>[2x]IQT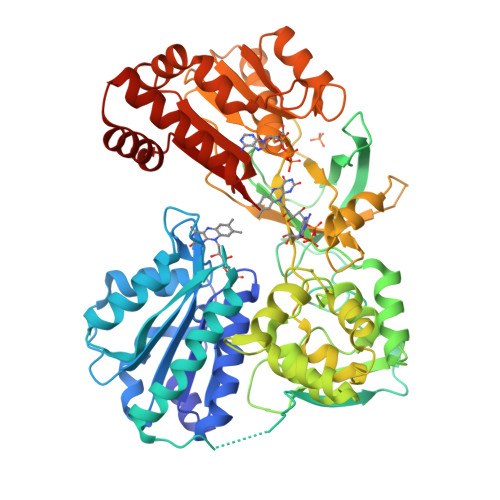TAPPVKESSFVEKMKKTGRNIIVFYGSQTGTAEEFANRLSKDAHRYGMRGMSADPEEYDLADLSSLPEIDKSLVVFCMATYEGDPTDNAQDFYDWLQETDVDLTGVKFAVFGLGNKTYEHFNAMGKYVDQRLEQLGAQRIFELGLGDDDGNLEEDFITWREQFWPAVCEFFGVEATGEESSIRQYELVVHEDMDVAKVYTGEMGRLKSYENQKPPFDAKNPFLAAVTANRKLNQGTERHLMHLELDISDSKIRYESGDHVAVYPANDSALVNQIGEILGADLDVIMSLNNLDEESNKKHPFPCPTTYRTALTYYLDITNPPRTNVLYELAQYASEPSEQEHLHKMASSSGEGKELYLSWVVEARRHILAILQDYPSLRPPIDHLCELLPRLQARYYSIASSSKVHPNSVHICAVAVEYEAKSGRVNKGVATSWLRAKEPAGENGGRALVPMFVRKSQFRLPFKSTTPVIMVGPGTGIAPFMGFIQERAWLREQGKEVGETLLYYGCRRSDEDYLYREELARFHKDGALTQLNVAFSREQAHKVYVQHLLKRDREHLWKLIHEGGAHIYVCGDARNMAKDVQNTFYDIVAEFGPMEHTQAVDYVKKLMTKGRYSLDVWS>APASLLPPAPEHSPPSSPLTQPPEGPKFPRVKNWEVGSITYDTLSAQAQQDGPCTPRRCLGSLVFPRKLQGRPSPGPPAPEQLLSQARDFINQYYSSIKRSGSQAHEQRLQEVEAEVAATGTYQLRESELVFGAKQAWRNAPRC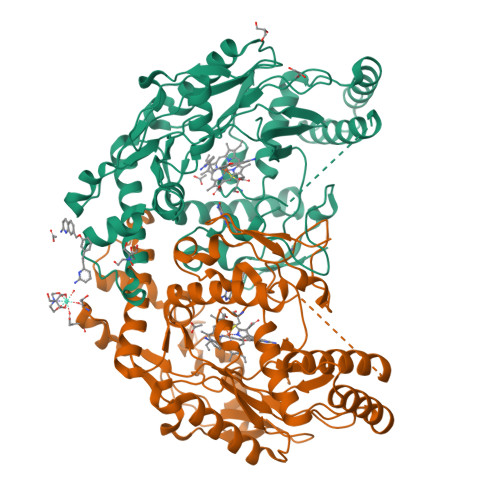VGRIQWGKLQVFDARDCRSAQEMFTYICNHIKYATNRGNLRSAITVFPQRCPGRGDFRIWNSQLVRYAGYRQQDGSVRGDPANVEITELCIQHGWTPGNGRFDVLPLLLQAPDEPPELFLLPPELVLEVPLEHPTLEWFAALGLRWYALPAVSNMLLEIGGLEFPAAPFSGWYMSTEIGTRNLCDPHRYNILEDVAVCMDLDTRTTSSLWKDKAAVEINVAVLHSYQLAKVTIVDHHAATASFMKHLENEQKARGGCPADWAWIVPPISGSLTPVFHQEMVNYFLSPAFRYQPDPW[2x]>MLIIETLPLLRQQIRRLRMEGKRVALVPTMGNLHDGHMKLVDEAKARADVVAVSIFVNPMQFDRPEDLARYPRTLQEDCEKLNKRKVDLVFAPSVKEIYPNGTETHTYVDVPGLSTMLEGASRPGHFRGVSTIV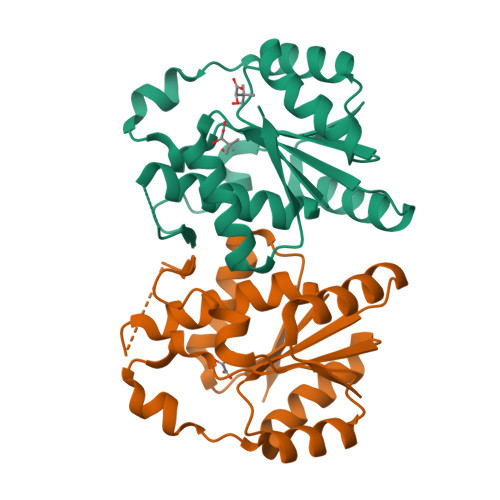SKLFNLVQPDIACFGEKDFQQLALIRKMVADMGFDIEIVGVP[2x]Botulinum neurotoxins (BoNTs) are produced by the anaerobic spore-forming bacteria Clostridium botulinum and cause neuromuscular paralysis (i.e., botulism) by proteolytic cleavage of SNARE (soluble N-ethylmaleimide-sensitive factor attachment protein receptor) proteins. All BoNTs are expressed as a single polypeptide chain that must be cleaved post-translationally to form the active di-chain molecule which is comprised of a 100 kDa heavy chain (HC) and 50 kDa light chain (LC). They all share a similar three-dimensional structure; the heavy chain folds into two distinct domains (the cell binding domain [HC] and the translocation domain [HN]), and the LC is a Zn2+-dependent metalloprotease. However, a BoNT-like gene (homologue of BoNT) was recently identified in the non-clostridial species, Enterococcus faecium, which is the leading cause of hospital-acquired multi-drug resistant infections. Interestingly, BoNT/En possesses the unique ability to cleave at least one member of all three SNARE-protein families (SNAP-25, VAMP, and STX); however, the cleavage of STX1 was only observed in vitro.

The structure of LC/En was determined at 2.0 Å with one molecule in the asymmetric unit by molecular replacement using the predicted structure from the AlphaFold2 server as a search model. Clear electron density was observed throughout the structure except for residues 127–130 and 249–260 which could not be modelled. The overall fold of LC/En is similar to all BoNT serotypes and homologues identified to date, consisting of a mixture of α-helices (31%) and β-strands (19%). The Zn2+ ion is coordinated by the HExxH motif residues, His225, Glu226 (via a bridged phosphate ion that has likely replaced the catalytic water molecule as observed in BoNT/A structure), His229, and an additional residue, Glu269 (inset). The analysis indicates that LC/En appears to have a much larger cleft volume than its closest related homologue, LC/X, and is most similar to LC/A. The presence of a glycine residue within the putative S1 subsite is particularly interesting as it would contribute to enhanced flexibility and reduced steric hindrance close to the catalytic zinc ion, such that it is less restricted by which substrate it can accommodate. Additionally, the lysine residues at positions 168 and 195 in place of hydrophobic residues (Phe163 and Phe194 in LC/A) within the S1′ subsite may further contribute to substrate promiscuity, given their increased length, rotamer angles, and potential ability to form both polar and non-polar contacts within the active site depending on the substrate. Loops 1 and 4 are significantly longer in LC/En compared to LC/A, LC/F, and LC/X. The additional portion of loop 1 contains several charged residues whereas loop 4 is predominantly hydrophilic, and the increased length of both loops may contribute to the substrate promiscuity observed for LC/En.

> MAHHHHHHSSGLEVLFQGMVTINDLHYSDPIDEDNIINMRIPLYDLEVDDQFINHNVPDLKAFQVFPNVWVVPERYTFYSTMKNLDAPANPSRSSYYDPTYLQSDAEKEVFLQQMILLFKRINSTQEGQQFLNLLSRSIPVPYESNGDVAMGTTQVIKQMDDKGNVLKHRRAHIIIYGPGPDLMAKGSKALTKSRETGRGCMAEIYFSPMYHKTYSTKLTNKNSLVDKSVQEFVPDPAVTLIHELCHGLHALYGIDLGNVGSWEFNSNPNSLFSSWFSSKEAVNFEEVMTFGGEDVKVIKSEIDKKIPGILNLIKTTVEPIINKITDPHDEMLQCLQSKYPSLKGTLGQFFFDDTQLEKDIRDLWMVMNETMFAENLKALTRARYLVPKVENIVQVDILSPNVYTIDKGFNHLSKGFKGQSVSQSYFRKISALARGAVVRACPQAF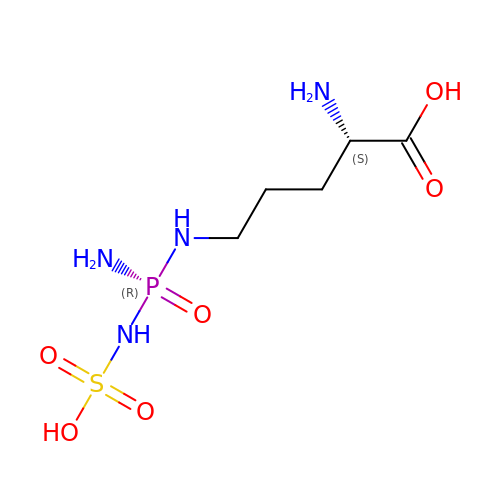NDELTA-(N'-SULPHODIAMINOPHOSPHINYL)-L-ORNITHINE | C5 H15 N4 O6 P S | MDGVOXPIIICZEK-FOIQGAMDSA-N> MTDDKDVLRDVWFGRIPTCFTLYQDEITEREAEPYYLLLPRVSYLTLVTDKVKKHFQKVMRQEDISEIWFEYEGTPLKWHYPIGLLFDLLASSSALPWNITVHFKSFPEKDLLHCPSKDAIEAHFMSCMKEADALKHKSQVINEMQKKDHKQLW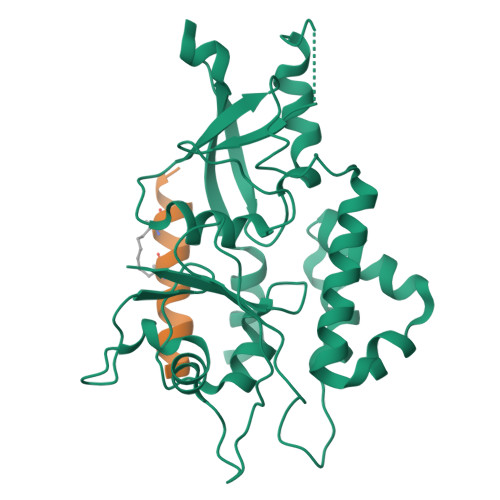MGLQNDRFDQFWAINRKLMEYPAEENGFRYIPFRIYQTTTERPFIQKLFRPVAADGQLHTLGDLLKEVCPSAIDPEDGEKKNQVMIHGIEPMLETPLQWLSEHLSYPDNFLHISIIPQPTD;> XWKRHISEQLRLRDRLQRQAFEX>[4x]TSEDACQDAEQPTRYETLFQALDRNGDGVVDIGELQEGLRNLGIPLGQDAEEKIFTTGDVNKDGKLDFEEFMKYLKDHEKKMKLAFKSLDKNNDGKIEASEIVQSLQTLGLTISEQQAELILQSIDVDGTMTVDWNEWRDYFLFNPVTDIEEIIRFWKHSTGIDI

The mitochondrial ATP-Mg/Pi carrier (APC) is a member of the mitochondrial carrier family of transport proteins. APC is involved in the import of cytosolic adenine nucleotides into the mitochondrion and the export of inorganic phosphate from the mitochondrial matrix. Therefore, APC has the important role of altering the mitochondrial adenine nucleotide pool in order to adapt to changing cellular energetic demands. The N-terminal domain of APC forms a calcium-sensitive regulatory domain.

The consequence of calcium binding to the regulatory domain of APC is a stimulation of the substrate transport activity of the carrier. A structure of the regulatory domain of human APC isoform-1 has recently been solved, confirming the presence of four EF-hands, each of which is occupied by a bound calcium ion in a canonical pentagonal bi-pyramidal fashion. The EF-hands group together into two pairs, forming two lobes connected by a long central α-helix, in a similar fashion to the four EF-hands of calmodulin. The linker region between the N-terminal regulatory domain and the C-terminal carrier domain contains an amphipathic α-helix of unknown function. In the structure this α-helix is bound to EF-hand pair 3 and 4, analogous to the binding of a calmodulin recognition sequence motif to the hydrophobic pockets in the EF-hands of calmodulin. The protein construct used in the previous study of the HsAPC-1 regulatory domain was mutated at the extreme N-terminus to replace a cysteine residue at position 15 with a serine, raising the possibility that a native dimer could have been disrupted. Therefore, the mechanism that couples calcium binding in the regulatory domain to substrate transport in the carrier domain has not been resolved. Here, an independent structural determination of the native human APC-1 regulatory domain was completed, which was combined with an investigation into the oligomeric state of the full-length human APC-1 protein. Furthermore, an extensive comparison of the conformations of EF-hand proteins in the calcium-free, calcium-bound and peptide-bound state was undertaken, which has allowed us to propose a mechanism for the regulation of APC that is consistent with all available experimental data.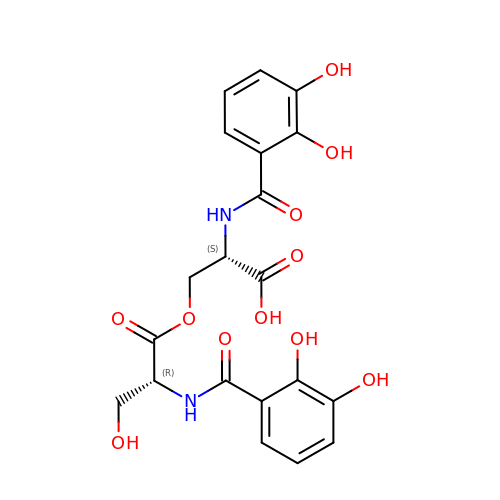N-[(2,3-dihydroxyphenyl)carbonyl]-O-[(2R)-2-{[(2,3-dihydroxyphenyl)carbonyl]amino}-3-hydroxypropanoyl]-L-serine | C20 H20 N2 O11 | KLXJDVFEFZPIMN-NEPJUHHUSA-N N-[2,4-bis(morpholin-4-yl)phenyl]-3-phenoxybenzamide | C27 H29 N3 O4 | 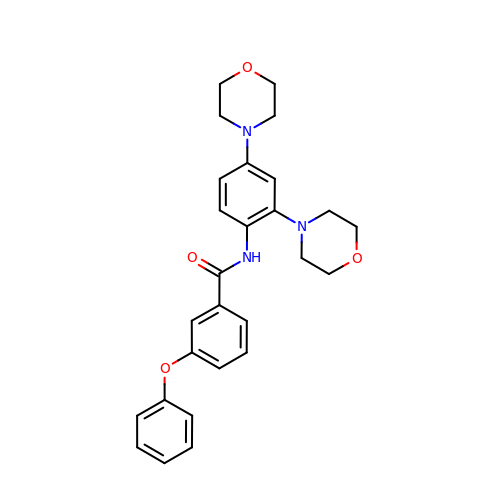NPIWJUNMCKXNKZ-UHFFFAOYSA-N> QSPPGKPEIHKCRSP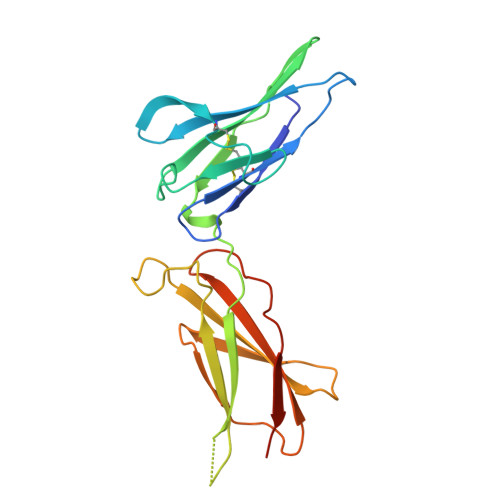DKETFTCWWNPGTDGGLPTNYSLTYSKEGEKTTYECPDYKTSGPNSCFFSKQYTSIWKIYIITVNATNQMGSSSSDPLYVDVTYIVEPEPPRNLTLEVKQLKDKKTYLWVKWSPPTITDVKTGWFTMEYEIRLKPEEAEEWEIHFTGHQTQFKVFDLYPGQKYLVQTRCKPDHGYWSRWSQESSVEMPNDFTLKD>TKCYNHQSTTPETTEICPDSGY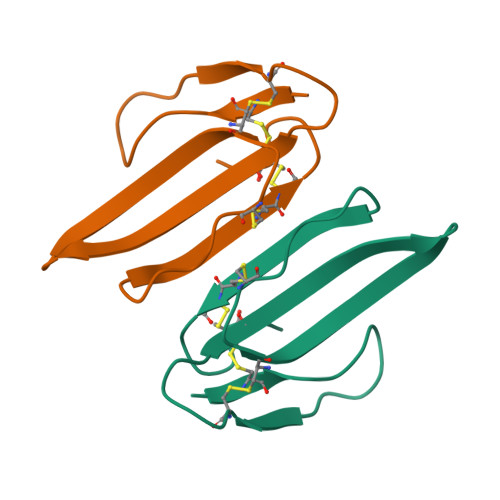FCYKSSWIDGREGRIERGCTFTCPELTPNGKYVYCCRRDKCNQ[2x]(1R)-2,2-DIMETHYL-1-({5-[4-(TRIFLUOROMETHYL)PHENYL]-1,3,4-OXADIAZOL-2-YL}METHYL)PROPYL 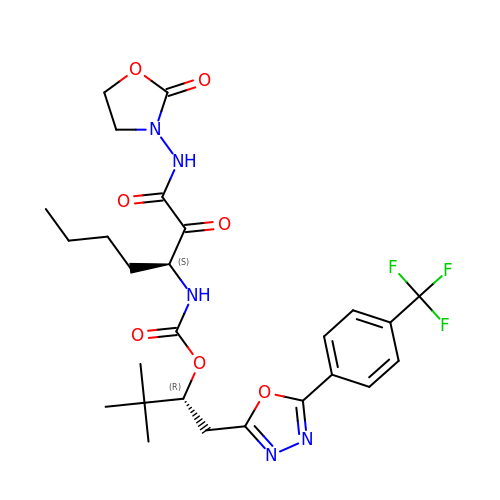(1S)-1-{OXO[(2-OXO-1,3-OXAZOLIDIN-3-YL)AMINO]ACETYL}PENTYLCARBAMATE | C26 H32 F3 N5 O7 | IXXKXSFSQVTOKQ-ZWKOTPCHSA-N> GDPVEDIIHDALGSTARRAISSATNVESAANTTPSSHRLETGRVPALQAAETGATSNATDENMIETRCVVNRNGVLETTINHFFSRSGLVGVVNLTDGGTDTTGYVTWDIDIMGFVQLRRKCEMFTYMRFNAEFTFVTTTKNGEARPYMLQYMYVPPGAPKPTGRDAFQ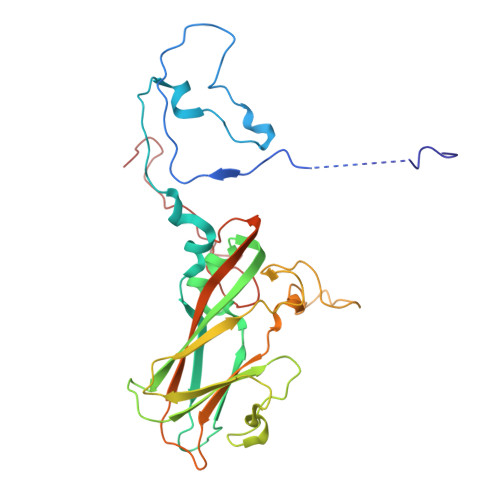WQTATNPSVFVKLTDPPAQVSVPFMSPASAYQWFYDGYPTFGQHPETSNTTYGLCPNNMMGTFAVRVVSREASQLKLQTRVYMKLKHVRAWVPRPIRSQPYLLKNFPNYDSSKITNSARDRSSIKQAN>[12x]MTPHINAKIGDF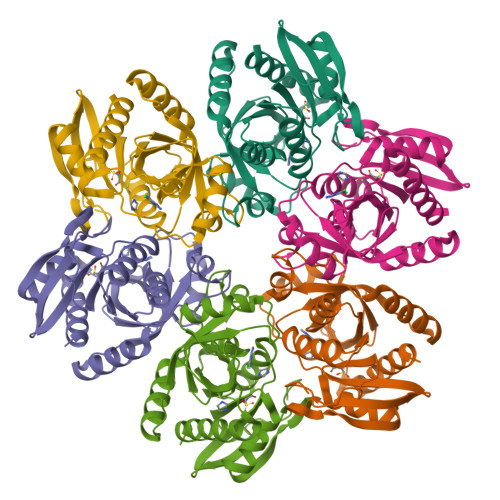YPQCLLCGDPLRVSYIAKKFLQDAKEITNVRNMLGFSGKYKGRGISLMGHGMGIASCTIYVTELIKTYQVKELLRIGTCGAISPKVGLKDIIMATGASTDSKTNRVRFLNHDLSATPDFELSLRAYQTAKRLGIDLKVGNVFSSDFFYSFETHAFDLMAKYNHLAIEMEAAGLYATAMELNAKALCLCSVSDHLITKEALSPKERVESFDNMIILALEMMS> MDTWMVLLGLQILLLPLLAHCTAPASTLRFVAVGDWGGVPNAPFHTAREMANAKEIARTVQIMGADFI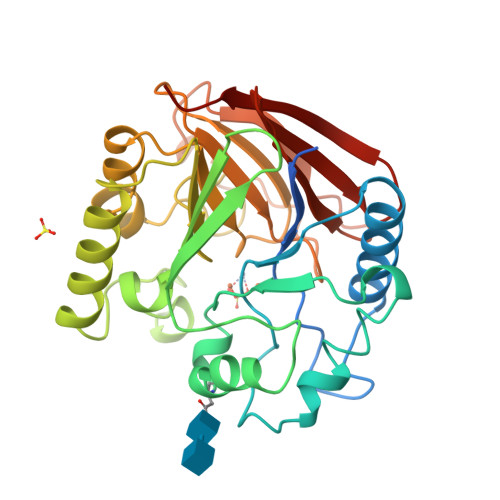MSLGDNFYFTGVHDANDKRFQETFEDVFSDRALRNIPWYVLAGNHDHLGNVSAQIAYSKISKRWNFPSPYYRLRFKVPRSNITVAIFMLDTVMLCGNSDDFVSQQPEMPRDLGVARTQLSWLKKQLAAAKEDYVLVAGHYPIWSIAEHGPTRCLVKNLRPLLAAYGVTAYLCGHDHNLQYLQDENGVGYVLSGAGNFMDPSVRHQRKVPNGYLRFHYGSEDSLGGFTYVEIGSKEMSITYVEASGKSLFKTSLPRRPRP> GAMERKANYAVDAYFREALRVSEPKAPKAPRPPKQPIVQDFQFFPPRLFELLDQEIYYFRKTVGYKVPKNTELGSDATKVQREEQRKIDEAEPLTEEEIQEKENLLSQGFTAWTKRDFNQFIKANEKYGRDDIDNIAKDVEGKTPEEVIEYNAVFWERCTEL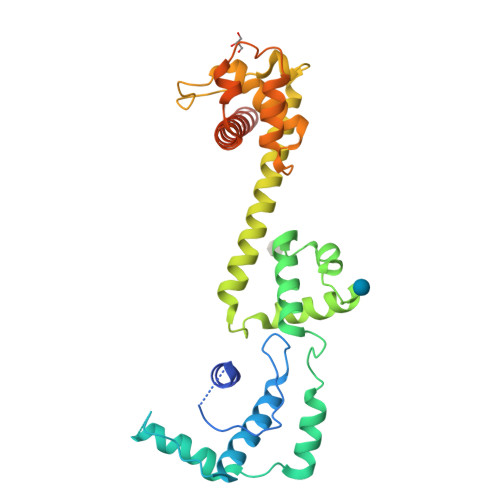QDIERIMGQIERGEGKIQRRLSIKKALDQKMSRYRAPFHQLRLQYGNNKGKNYTEIEDRFLVCMLHKLGFDKENVYEELRAAIRASPQFRFDWFIKSRTALELQRRCNTLITLIERENIELEEKERAEKKKKAPKGSVSAGS> MLKKLFGAKKEFYVQLDESQAPA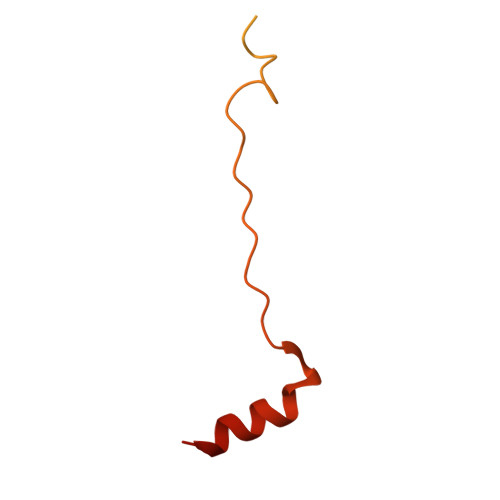QVEEADVAIVKSEVAPVEKPAPTTSKKTSIKKKSATKAAAPVETPASAPVAPAPKAKVDPSQVAFASGDPIPQNVARRTPGPSLNRFKEMARQVKVKR>MGSSHHHHHHSSGLEVLFQGPAERISKQSTPFVGAQIFIEPGQTQEQIEQWFKLLAESNMTTCRIRMFGKYMKTPSGTYDFTLFDRAFKLADKYHIKVYATLFPDTEFTDVGGFKFPHSREHQKEVEDYIKNVVSHFSQYKNLAAWVLINEPGTPNLPFNEPFTKERFSDWKKEHNFSEYNEKGYPVLNFEKENFIIDYHNWYLNWLANQVRLYDKQHDLHVNPHNVFKLSGLYDFPTWRTFLNSLGGSAHASWHFGYFPRKAYTVAMSANAELIRSGAGELPWLMTELQGGNNLYSGANPLCPTAEEIIQWLWINFATEAKGGIFWSFNARSTAAEAGEWAMINFKNKSSDRLIAAATIGKFITENVKMMSNIKTLNSGISILYNHESMWVEAAQTRGKLNGNGRSIGAVMCSPLSYFEALSETGLQANFKEIKEFDFSLNDYTDQVIILSHQIALDNKVIKQLESFVEKGGTLIADGLTGYYDYQAHSTVVSGFALENLFGSYPIEYKIKENLFSLDFEKDNYKLPAHLWKGTIETSKATPIMDKEGECIACINQYGKGKVFWIPSPIALGARESKDFSELSKLTVSLLPNKILNDNPHFDKHYKDVMMKSFKSNGTMYSLIINKSASVQTVDIVGGKGKAFILFANKNAHSTANKLTISPEETVIIKWKNN[6x]

Exo-β-mannosidases, hydrolysing non-reducing terminal β-d-mannopyranosidic linkages, are widely distributed carbohydrate-degrading enzymes. All of these exo-β-mannosidases process their substrate using a stereochemically retaining double displacement mechanism that is characterised by the formation of a covalent glycosyl enzyme intermediate (GEI). We show that these probes covalently label exo-β-mannosidases from GH families 2, 5, and 164. Structural studies of the resulting complexes support a canonical mechanism-based mode of action in which the active site nucleophile attacks the pseudoanomeric centre to form a stable ester linkage, mimicking the glycosyl enzyme intermediate.

BsGH164 did not react with N-octylazido aziridine 3, but was labelled by both epoxide 1 (76% inhibition) and aziridine 2 (30% inhibition). Soaking BsGH164 crystals with 1 or 2 (1 mM, 3 days, RT, pH 6.5) resulted in the formation of clear covalent adducts. Both complexes have the ligand in the same position, sharing a 4C1/E5 conformation as observed for the complex with 2FMan (ESI Fig. 4†).5 H260 shows a slight displacement in the complex with compound 2. The structure presents no obvious basis for the lack of reactivity with compound 3 as the pocket is quite open around the aziridine nitrogen. In fact, an ethylene glycol monomer is observed bound where the linker could reasonably be accommodated. Our structural work shows that the epoxide and aziridine inhibitors bind BsGH164 in the same conformation found as 2FMan and that the N-alkyl aziridine binds to CmMan5A in the expected OS2-like conformation of the GH5 exo-β-mannosidase GEI.> MNKHSGIDFKQLNFLTKLNENHSGELWKGRWQGNDIVVKVLKVRDWSTRKSRDFNEECPRLRIFSHPNVLPVLGACQSPPAPHPTLITHWMPYGSLYNVLHEGTNFVVDQSQAVKFALDMARGMAFLHTLEPLIPRHALNSRSVMIDEDMTARISMADVKFSFQSPGRMYAPAWVAPEALQKKPEDTNRRSADMWSFAVLLWELVTREVPFADLSNMEIGMKVALEGLRPTIPPGISPHVSKLMKICMNEDPA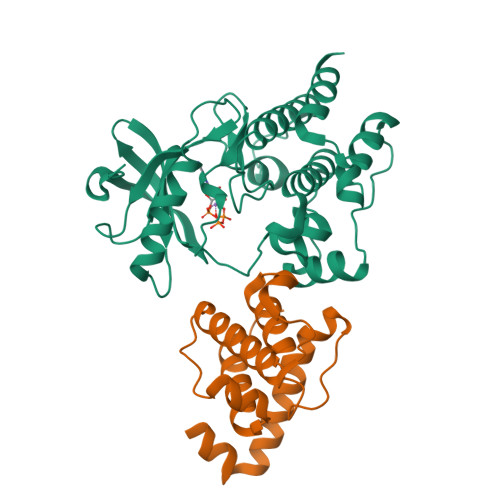KRPKFDMIVPILEKMQDK;> GSHMDAFDTLFDHAPDKLNVVKKTLITFVNKHLNKLNLEVTELETQFADGVYLVLLMGLLEGYFVPLHSFFLTPDSFEQKVLNVSFAFELMQDGGLEKPKPRPEDIVNCDLKSTLRVLYNLFTKYRNVE The main pathway for ethanol production in C. thermocellum involves the bifunctional aldehyde-alcohol dehydrogenase (AdhE). AdhE functions in the anaerobic fermentation pathway and contains two domains: an aldehyde dehydrogenase (ALDH) domain for the reduction of acetyl-CoA to acetaldehyde and an alcohol dehydrogenase (ADH) domain to reduce acetaldehyde to ethanol. Both reduction processes natively use NADH as a cofactor and are reversible in the presence of NAD+ as a cofactor. Structurally, AdhE is an intriguing protein as it forms large, filamentous helical ultrastructures termed spirosomes, that could be necessary for function.

Using standard cryo-EM techniques, we were able to determine a 3.28 Å cryo-EM structure of the extended C. thermocellum AdhE spirosome. We determined that the native state of the C. thermocellum spirosome is extended (different from that of other structurally characterized AdhEs) and contains an enclosed channel between the ALDH and ADH active sites. The first is the buried area located between two molecules of AdhE, in a domain-swapped dimer interface, where one ALDH domain is sandwiched between the ADH and ALDH domains of the second protein. The second interface is between the dimer of dimers, here referred to as the tetramer interface. This interface has a much smaller interaction area because it only occurs between two ADH domains. However, the calculated buried surface area differs between the two E. coli dimer interfaces, but not the tetramer interface. Both the E. coli and C. thermocellum extended dimer interfaces bury ~5000 Å2. We found that more salt bridges form in the extended C. thermocellum structure as compared to the extended E. coli structure, which suggests that this may be a factor in the stability of the extended C. thermocellum structure that is not found in the E. coli structure. At the ADH active site, we observe an empty density in the C. thermocellum extended structure, coordinated between residues that have been implicated in the ADH activity of the protein (circled in red). We see that there is density, most probably a water molecule, being coordinated by H734, D844, and C846. While the channel can be found in both the compact and extended structures, we see that the channel in the compact conformation has areas that are exposed to the cytosol, whereas the extended channel is entirely enclosed.

>[6x]MHHHHHHENLYFQGMTKIANKYEVIDNVEKLEKALKRLREAQSVYATYTQEQVDKIFFEAAMAANKMRIPLAKMAVEETGMGVVEDKVIKNHYASEYIYNAYKNTKTCGVIEEDPAFGIKKIAEPLGVIAAVIPTTNPTSTAIFKTLIALKTRNAIIISPHPRAKNSTIEAAKIVLEAAVKAGAPEGIIGWIDVPSLELTNLVMREADVILATGGPGLVKAAYSSGKPAIGVGAGNTPAIIDDSADIVLAVNSIIHSKTFDNGMICASEQSVIVLDGVYKEVKKEFEKRGCYFLNEDETEKVRKTIIINGALNAKIVGQKAHTIANLAGFEVPETTKILIGEVTSVDISEEFAHEKLCPVLAMYRAKDFDDALDKAERLVADGGFGHTSSLYIDTVTQKEKLQKFSERMKTCRILVNTPSSQGGIGDLYNFKLAPSLTLGCGSWGGNSVSDNVGVKHLLNIKTVAERRENMLWFRTPEKIYIKRGCLPVALDELKNVMGKKKAFIVTDNFLYNNGYTKPITDKLDEMGIVHKTFFDVSPDPSLASAKAGAAEMLAFQPDTIIAVGGGSAMDAAKIMWVMYEHPEVDFMDMAMRFMDIRKRVYTFPKMGQKAYFIAIPTSAGTGSEVTPFAVITDEKTGIKYPLADYELLPDMAIVDADMMMNAPKGLTAASGIDALTHALEAYVSMLATDYTDSLALRAIKMIFEYLPRAYENGASDPVAREKMANAATIAGMAFANAFLGVCHSMAHKLGAFYHLPHGVANALMINEVIRFNSSEAPTKMGTFPQYDHPRTLERYAEIADYIGLKGKNNEEKVENLIKAIDELKEKVGIRKTIKDYDIDEKEFLDRLDEMVEQAFDDQCTGTNPRYPLMNEIRQMYLNAYYGGAKK>MGSMEFVNKQFNYKDPVNGVDIAYIKIPNAGQMQPVKAFKIHNKIWVIPERDTFTNPEEGDLNPPPEAKQVPVSYYDSTYLSTDNEKDNYLKGVTKLFERIYSTDLGRMLLTSIVRGIPFWGGSTIDTELKVIDTNCINVIQPDGSYRSEELNLVIIGPSADIIQFECKSFGHEVLNLTRNGYGSTQYIRFSPDFTFGFEESLEVDTNPLLGAGKFATDPAVTLAHQLIYAGHRLYGIAINPNRVFKVNTNAYYEMSGLEVSFEELRTFGGHDAKFIDSLQENEFRLYYYNKFKDIASTLNKAKSIVGTTASLQYMKNVFKEKYLLSEDTSGKFSVDKLKFDKLYKMLTEIYTEDNFVKFFKVLNRKTYLNFDKAVFKINIVPKVNYTIYDGFNLRNTNLAANFNGQNTEINNMNFTKLKNFTGLFEFYKLLCVDGGGGSGGGGSGGGGSEMDENLEQVSGIIGNLRHMALDMGNEIDTQNRQIDRIMEKADSNKTRIDEANQRATKMLGSGANSALAGGGGSGGGGSGGGGSLQCIKVNNWDLFFSPSEDNFTNDLNKGEEITSDTNIEAAEENISLDLIQQYYLTFNFDNEPENISIENLSSDIIGQLELMPNIERFPNGKKYELDKYTMFHYLRAQEFEHGKSRIALTNSVNEALLNPSRVYTFFSSDYVKKVNKATEAAMFLGWVEQLVYDFTDETSEVSTTDKIADITIIIPY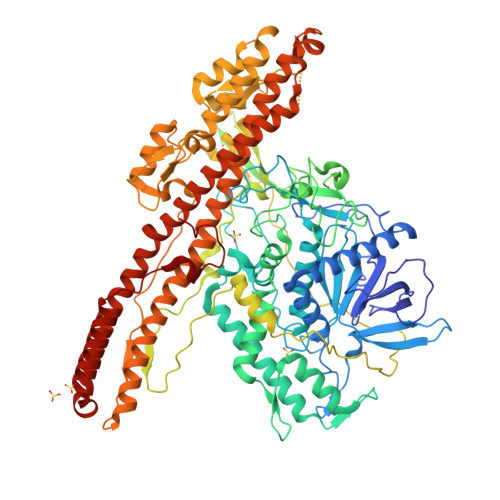IGPALNIGNMLYKDDFVGALIFSGAVILLEFIPEIAIPVLGTFALVSYIANKVLTVQTIDNALSKRNEKWDEVYKYIVTNWLAKVNTQIDLIRKKMKEALENQAEATKAIINYQYNQYTEEEKNNINFNIDDLSSKLNESINKAMININKFLNQCSVSYLMNSMIPYGVKRLEDFDASLKDALLKYIYDNRGTLIGQVDRLKDKVNNTLSTDIPFQLSKYVDNQRLLSTLEAHHHHHHHHHH[2x]>[12x]MAATSGFAGAIGQKLPPFSYAYTELEAI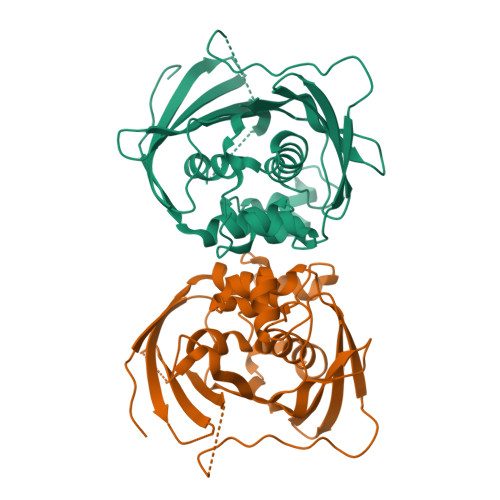MYALGVGASIKDPKDLKFIYEGSSDFSCLPTFGVIIGQKSMMGGGLAEIPGLSINFAKVLHGEQYLELYKPLPRAGKLKCEAVVADVLDKGSGVVIIMDVYSYSEKELICHNQFSLFLVGSGGFGGKRTSDKVKVAVAIPNRPPDAVLTDTTSLNQAALYRLSGDWNPLHIDPNFASLAGFDKPILHGLCTFGFSARRVLQQFADNDVSRFKAVKARFAKPVYPGQTLQTEMWKEGNRIHFQTKVQETGDIVISNAYVDLAPTSGTSAKL>GAADKRIDGNGNPETREIKISDYDEITFVGSADFEYEQSDKAPYLSVTIDENLFDYLVTEVEGGTLKIYPKSIKKGFNNNSYDLRPTVYKIKSNSKELKELNTVGSGSFIISKPTKVNRMEINMAGSGNVELR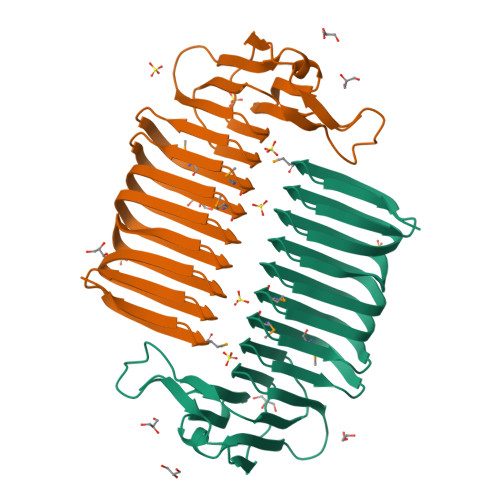GPVKGYKLECNMAGSGNIIAKDIQLDNLSCSLASSGEIEVIGTVDRASFNVAGSGEIKAFDCQARKAECNIASSGEISVYATQILDANIVGSGEIHYKGDPEISKSIMGSGSINKVK[6x]> AGGGT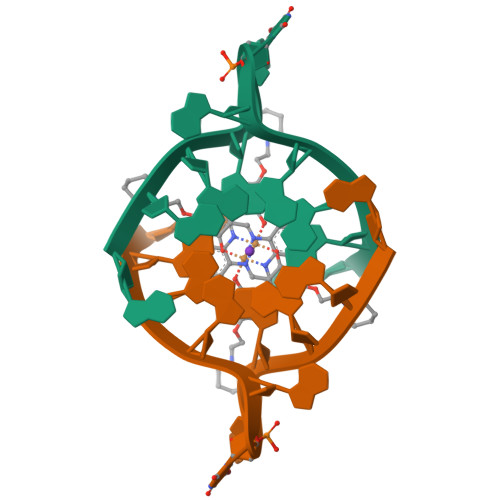UAGGGTT>MSEIGTGFPFDPHYVEVLGSRMHYVDVGPRDGTPVLFLHGNPTSSYLWRNIIPHVAPSHRCIAPDLIGMGKSDKPDLDYRFDDHVRYLDAFIEALGLEEVVLVIHDWGSALGFHWAKRNPERVKGIAFMEFIRPIPTWDEWPEFARELFQAFRTPDVGRELIIDQNAFIEGILPKFVVRPLTEVEMDHYREPFLKPVWREPLWRFPNELPIAGEPANIWALV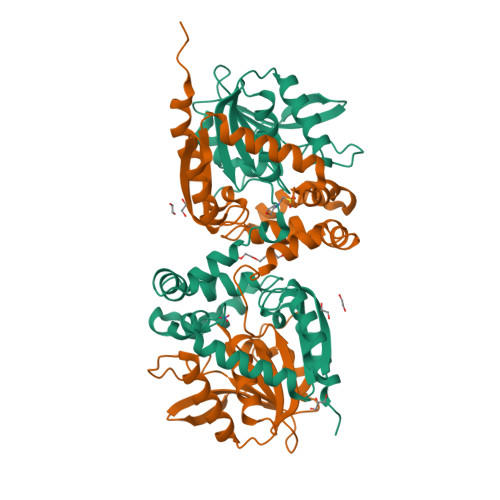EAYMNWLHQSPVPKLLFWGTPGVLIPPAEAARLAESLPNLKTVFIGPGLHYLQEDNPDLIGSEIARWLPALHHHHHH[2x]The enzyme is serving as a terminase in anaerobic glycolysis pathway, which performs the reversible catalysis from pyruvate to lactate, with nicotinamide adenine dinucleotide (NAD+) and its reduced form (NADH) as coenzymes (Dando et al., 2001). Apicomplexan parasites rely on anaerobic metabolism to produce ATP for various biochemical processes, and these protozoal LDHs have been considered as ideal potential targets for diagnosis and drug screening (Piper et al., 1999; Dando et al., 2001; Al-Anouti et al., 2004; Cornillot et al., 2012; Witola et al., 2017). BoLDH is a tetrameric enzyme made of four identical subunits and displays 222 (D2) symmetry. Taken together, the studies indicate that Babesia spp. LDHs could serve as a potential drug target for the development of anti-babesial compounds.

The crystal structure of BoLDH apo form (residues Met1 to Gly330) was determined by molecular replacement method and refined to R work and R free factors of 0.236/0.268 using reflections to 2.67 Å resolution (resolution range, 44.11–2.67 Å). The BoLDH crystals belong to the space group P1 with the unit cell parameters a = 81.9, b = 92.3, and c = 109.9 (Å). Two tetramers were observed per asymmetric unit, and each monomer contains a co-factor binding site for the binding of NADH or NAD+ and a substrate binding site for the binding of pyruvate or lactate. As the active-site loop (residues 95–109) in open and disordered state, a poor electron density map for the loop was displayed. In addition, an extra insertion (position 101–105, —DEEWS—) is present in the active-site loop (β4–α3 loop) of BoLDH and creates a larger catalytic pocket than that of mammalian LDHs. Interestingly, the absence of this five-peptide insertion makes the BoLDH lose its catalytic function. An extension of ~15 residues at the N-terminal, named as N-terminal “arm”, was detected in the apo BoLDH structure, and each “arm” was involved in the formation of an extra salt bridge in the way that a proton transfers from the carboxyl group of residue Asp266 to the guanidine group of residue Arg15 at the interface of subunit A and subunit C or subunit B and subunit D. The results together suggest that the N-terminal “arm” structure is contributed to the quaternary stabilization of BoLDH but not an essential factor for the stabilization of R-state conformation. Interestingly, we found that the structure of apo BoLDH takes R state with the active-site loop (β4–α3 loop) open, and the feature is similar to other eukaryotic apo LDHs, such as PfLDH, HuLDH-A, and BmLDH, but obviously different from that of bacterial LDHs in R state with the active-site loop closed. Hence, BoLDH belongs to a group of non-allosteric L-LDHs.

>[8x]MLKGFLSTMSPAVRRNKISLIGAGNIGGVMAYLAQLKELGDVVLFDIAPKLGEAKALDIMHANAIYDTAHKAIGTANYEDIADSDVCIITAGLAKLPNKKDEEWSRDDLVAPNSKIMFTIGDNIKKYAPNAFVICITNPLDVMVKMLLKATGFPKNKVVGMGGLLDSSRMCHYIADKLNVNPRYVHGSCIGGHGDSMIPLVNHVTVNGIPIQLFVERGDITQAELDKIAQRTIGSGMELVQLYGNGSAYFAPATAAIEMASAYLNDKKSVIVCSCYLEGEYGHSDVYLGTPAIIGANGIEKIITLKLSSEEQAKLDASVKEIMRLEALAG> GPVDSTDVRRITPKKLRELSDLLR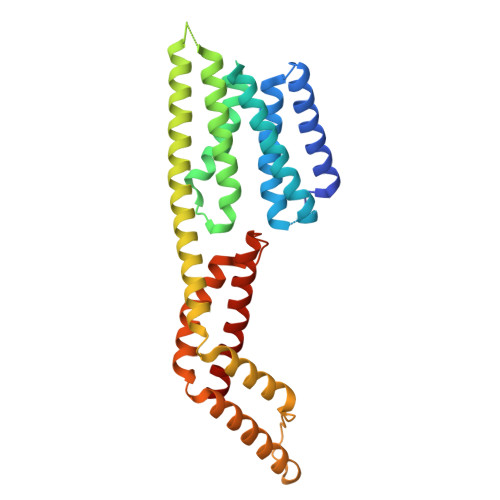THLSSAATKQLDMGGVLSDLDTMLVALDKAEREGGVDKDQLKSFNSLILKTYRVIEDYVKGREGDTKNSSTEVSPYHRSNFMLSIVEPSLQRIQKHLDQTHSFSDIGSLVRAHKHLETLLEVLVTLSQQGQPVSSETYGFLNRLAEAKITLSQQLNTLQQQQESAKAQLSILINRSGSWADVARQSLQRFDSTRPVVKFGTEQYTAIHRQMMAAHAAITLQEVSEFTDDMRNFTVDSIPLLIQLGRSSLMDEHLVEQREKLRELTTIAERLNRLEREWM>[8x]MEPTTEIQATEDLTLSGDHAAASADSLVVDNANDNAGQEEGFEIVLKDDETAPKQDPAKNAEFARRRIERKRQRELEQQMEAVKRGELPESLRVNPDLPPQPDINAYLSEEGLAKYDYDNSRALAAFNAANTEWLMKAQDARSNAVAEQGRKTQEFTQQSAQYVEAARKHYDA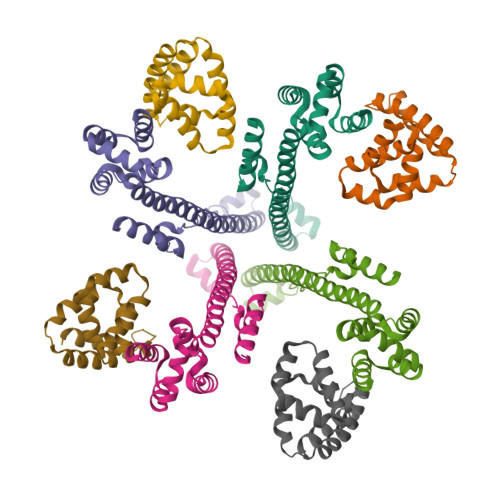AEKLNIPDYQEKEDAFMQLVPPAVGADIMRLFPEKSAALMYHLGANPEKARQLLAMDGQSALIELTRLSERLTLKPRGKQISSAPPADQPITGDVSAANKDAIRKQMDAAASKGDVETYRKLKAKLKGIR> SATEPPKIVWNEGKRRFETEDHEAFIEYKMRNNGKVMDLVHTYVPSFKRGLGLASHLCVAAFEHASSHSISIIPSCSYVSDTFLPRNPSWKP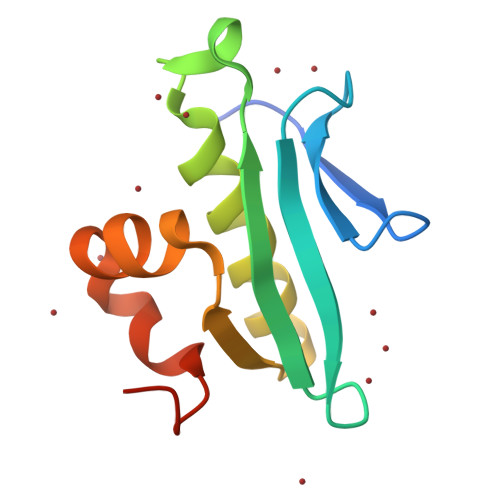LIHSEVFKSSI>[2x]MGGSEYRVDLVVLSEQKQNCRFGLTFHNLSDQDLNSWGLTFAFDRYILPDSVSNGQLTQIGSFCTLKPEGIVLAANHHYYCEFSIGSNPFRYYSDGFNEAMIDFVVDGQPQRAQVDVTPIVLASPYRERSDIPASLTHAQPLLPKPNHIEVSDHSFTFDEQAGVAIYTDLANSAKAWLLEELQRIHQFTLSSSNSGKIIFKSNPTLDEGAYKLKVSEESIKIEAGSSSGFTHACATLLQLLKRDEATKTMEAVCCSIIDSPRFRYRGMMLDCARHFHSVEQVKRLINLLAHYKLNTFHWHLTDDEGWRVEIKSLPQLTEIGAWRGIDETIEPQYTHLSQRYGGFYTQEEIRDVIAFAEQRGITIIPEIDVPGHCRAAIKSLPHLLIEAEDTTEYRSIQHYNDNVINPALPGSYEFIDKVLEEIAALFPAPYVHIGADEVPNGVWSKSPACQALMEQLGYTDYKELQGHFLRHAEDKLRKLGKRMLGW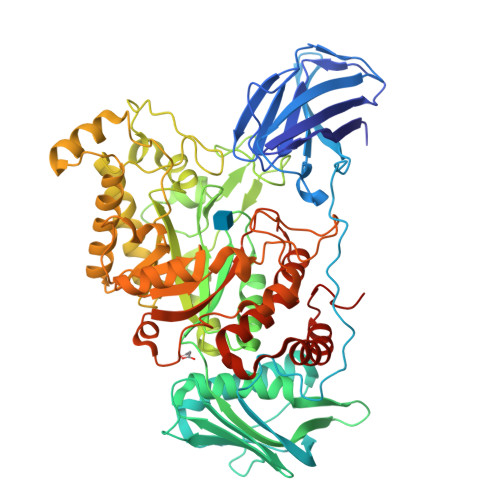EEAQHGNKVSKDTVIYSWLSEEAALNCARQGFDVVLQPAQTTYLDMTQDYAPEEPGVDWANPLPLEKAYNYEPLAEVPADDPIRKRIWGIQTALWCEIINNPSRMDYMIFPRLTAMAEACWTEKQHRDWTDYLSRLKGHLPLLDLQGVNYRKPWKRSRSHHHHHH(4S,6S)-6-{[(3R,4R)-4-{2-[(2,2-difluoro-2-phenylethyl)amino]ethoxy}pyrrolidin-3-yl]methyl}-4-methyl-3,4,5,6-tetrahydropyridin-2-amine | C21 H32 F2 N4 O | 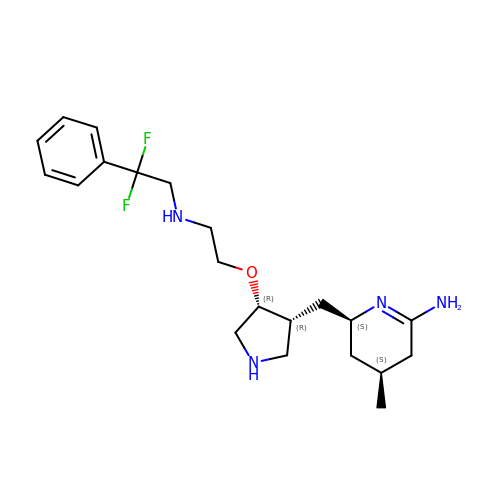DAHQXGAQQOLJFX-NBMJBFSESA-N>[2x]MPLVSMKEMLIDAKENGYAVGQYNINNLEFTQAILEASQEENAPVILGVSEGAARYMSGFYTIVKMVEGLMHDLNITIPVAIHLDHGSSFEKCKEAIDAGFTSVMIDASHSPFEENVATTKKVVEYAHEKGVSVEAELGTVGGQEDDVVADGIIYADPKECQ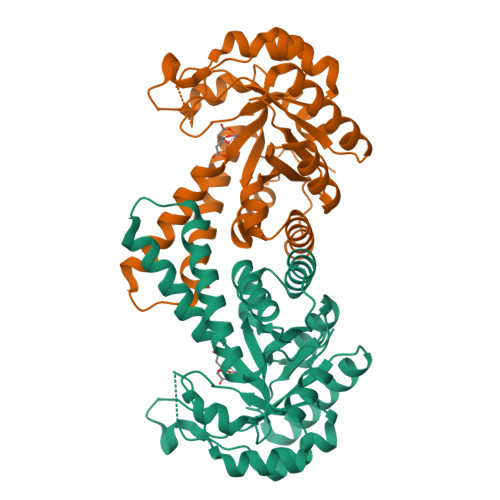ELVEKTGIDALAPALGSVHGPYKGEPKLGFKEMEEIGLSTGLPLVLHGGTGIPTKDIQKAIPFGTAKINVNTENQIASAKAVRDVLNNDKEVYDPRKYLGPAREAIKETVKGKIKEFGTSNRAKHHHHHH> MMINIQEDKLVSAHDAEEILRFFNCHDSALQQEATTLLTQEAHLLDIQAYRAWLEHCVGSEVQYQVISRELRAASERRYKLNEAMNVYNENFQQLKVRVEHQLDPQNWGNSPKLRFTRFITNVQAAMDVNDKELLHIRSNVILHRAR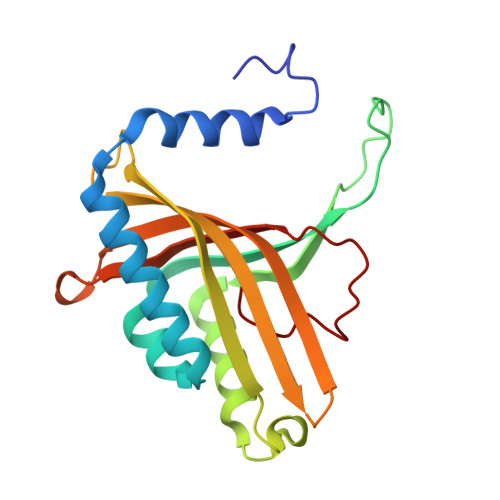RGNQVDVFYAAREDKWKRGEGGVRKLVQRFVDYPERILQTHNLMVFL> GPGSVDTERPVVDFPGEINVYRGESFEFIATATDNSNAFDINKTYVRWYNGTDSGRGTEWIEKTVTQEGNLLKVKVHGKVPVDTDIGHYTRYVMVTDAAGNQNVSNEEFSAALTNKDRILNGQFRIVIRYRPNLPENTVLVNNPSQLSE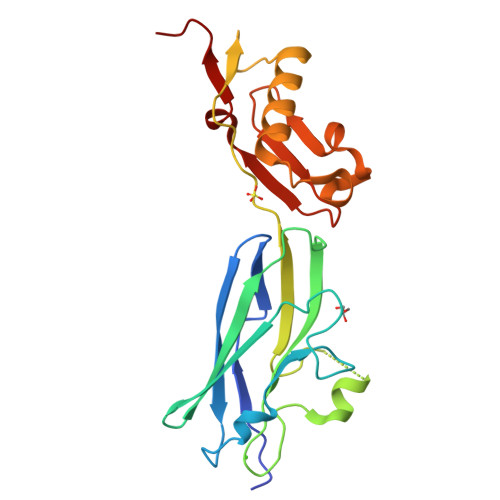TEKNQVREAIKQSNPNLRPIDVAGKNLDTAISVSNNGTTTITFRDNRKATIQGKDLVDTRAGS>[4x]GCGGGTSTQGSESSSGGDASGSYDVSSQSITFIPKQLNNPFSDVMLGGGKNAAGEIGFAEVNVVGPLEASSSSQVSFINSEVQAGTNVLVIAANDPDAVCPALQDARKAGTKVVTFDSDSAADCRDLFINQVESKQVAITMLDMVSDQIGGSGKVAILSATANAANQNAWIKFMEDEIASNDKYKGIEIVAKVYGDDDDTKSFQEAQGLLQAHPDLNAIVSPTTVGIAATA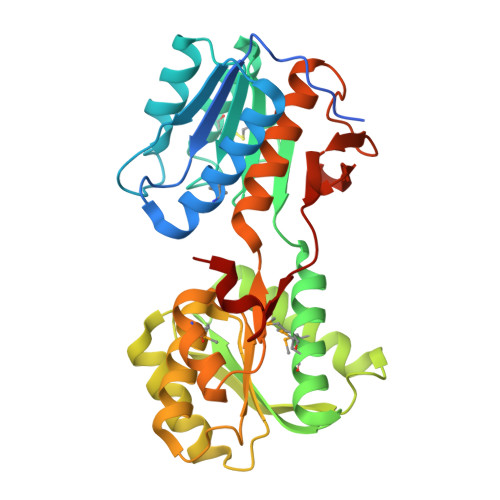RYLSTSDYKGKVFLTGLGLPNEMRSFVKDGTVKEFALWDPAQLGYVAAYAGAALDSGAIKGEVGEKFTAGNLGERTIGENKTVVVGDPVRFNADNIDKYDF> HSWRHIRAEGLDSSYTVLFGKAEADEIFQELEKEVEYFTGALARVQVFGKWHSVPRKQATYGDAGLTYTFSGLTLSPKPWIPVLERIRDHVSGVTGQTFNFVLINRYKDGSDHICEHRDDERELAPGSPI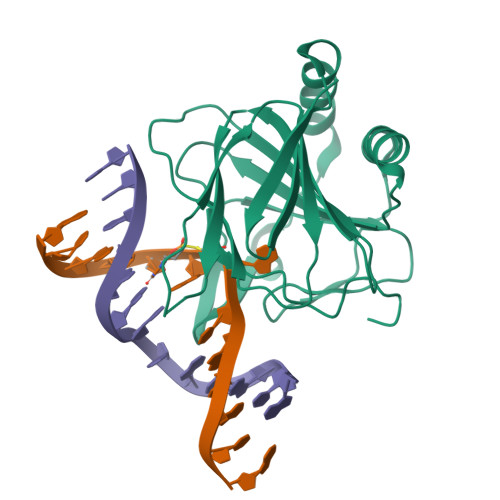ASVSFGASRDFVFRHKDSRGKSPSRRVAVVRLPLAHGSLLMMNHPTNTHWYHSLPVRKKVLAPRVNLTFRKILLTA N'-acetyl-2-[(3R)-1,1-dioxo-1lambda~6~-thiolan-3-yl]acetohydrazide | C8 H14 N2 O4 S | 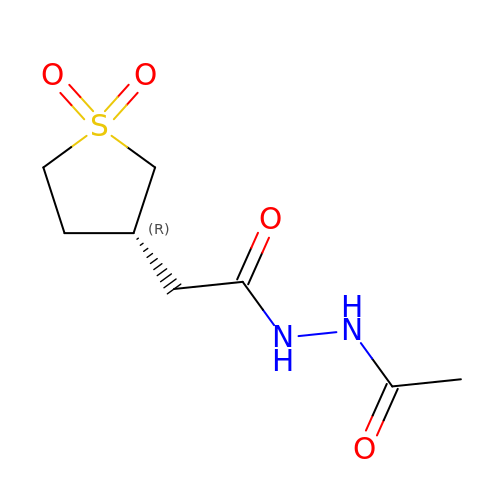DIHAZQXZGGBQIS-ZETCQYMHSA-N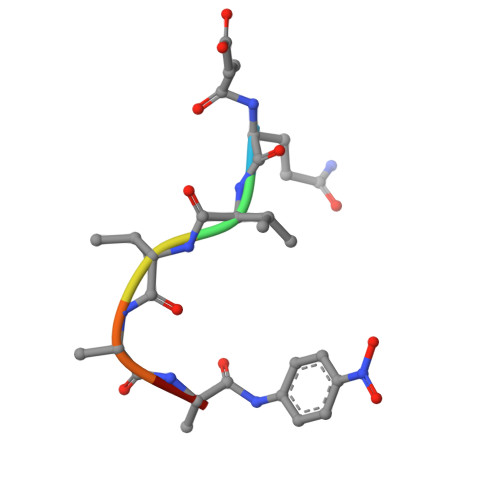> QVVAAX>[10x]DYKDDDDKLHSQANLMRLKSDLFNRSPMYPGPTKDDPLTVTLGFTLQDIVKA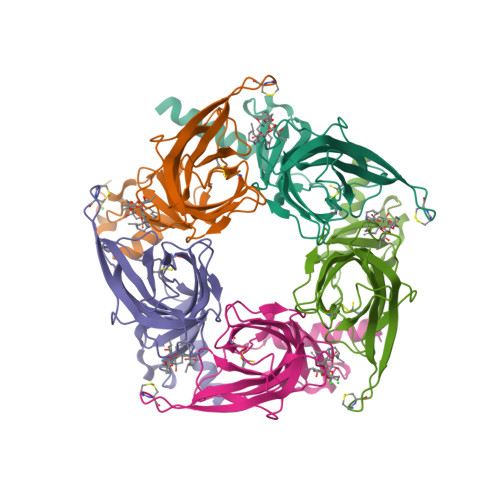DSSTNEVDLVYYEQQRWKLNSLMWDPNEYGNITDFRTSAADIWTPDITAYSSTRPVQVLSPQIAVVTHDGSVMFIPAQRLSFMCDPTGVDSEEGATCAVKFGSWVYSGFEIDLKTDTDQVDLSSYYASSKYEILSATQTRQVQHYSCCPEPYIDVNLVVKFRERR> MGLTNRLNATSNYSEYSLSVAVLADSEIENVTQLTSVTAPTGTDNENIQKLLADIKSSQNTDLTVNQSSSYLAAYKSLIAGETKAIVLNSVFENIIELEYPDYASKIKKIYTKGFTKKVEAPKTSKNQSFNIYVSGIDTYGPISSVSRSDVNILMTVNRDTKKILLTTTPADAYVPIADGGNNQKDKLTHAGIYGVDSSIHTLENLYGVDINYYVRLNFTSFLKMIDLLGGVDVHNDQEFSALHGKFHFPVGNVHLDSEQALGFVRERYSLADG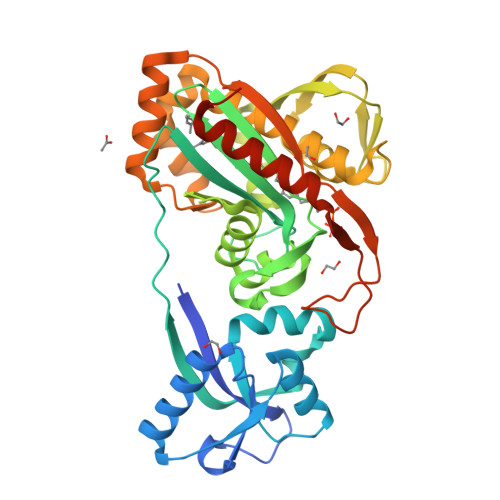DRDRGRNQQKVIVAILQKLTSTEALKNYSTIINSLQDSIQTNVPLETMINLVNAQLESGGNYKVNSQDLKGTGRMDLPSYAMPDSNLYVMEIDDSSLAVVKAAIQDVMEGRKLAAALEHHHHHH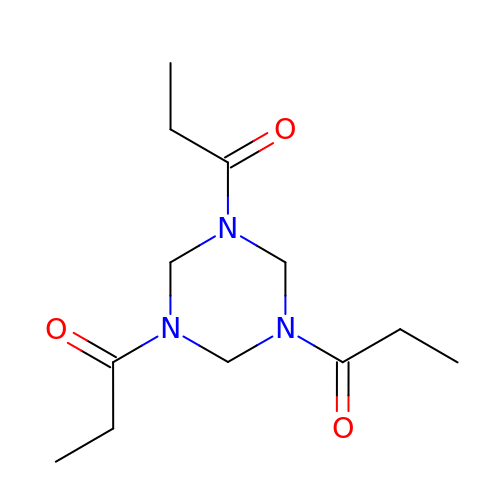1,1',1''-(1,3,5-triazinane-1,3,5-triyl)tripropan-1-one | C12 H21 N3 O3 | AEPJNZPJFYDQLM-UHFFFAOYSA-N>MIHHHHHHEHRHLKPFPPEFLWGAASAAYQVEGAWNEDGKGLSVWDVFAKQPGRTFKGTNGDVAVDHYHRYQEDVALMAEMGLKAYRFSVSWSRVFPDGNGAVNEKGLDFYDRLIEELRNHGIEPIVTLYHWDVPQALMDAYGAWESRRIIDDFDRYAVTLFQRFGDRVKYWVTLNEQNIFISFGYRLGLHPPGVKDMKRMYEANHIANLANAKVIQSFRHYVPDGKIGPSFAYSPMYPYDSRPENVLAFENAEEFQNHWWMDVYAWGMYPQAAWNYLESQGLEPTVAPGDWELLQAAKPDFMGVNYYQTTTVEHNPPDGVGEGVMNTTGKKGT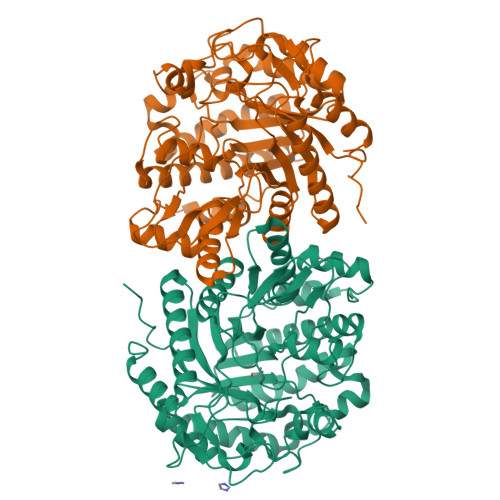STSSGIPGLFKTVRNPHVDTTNWDWAIDPVGLRIGLRRIANRYQLPILITENGLGEFDTLEPGDIVNDDYRIDYLRRHVQEIQRAITDGVDVLGYCAWSFTDLLSWLNGYQKRYGFVYVNRDDESEKDLRRIKKKSFYWYQRVIETNGAEL[2x]> MPVDFTGYWKMLVNENFEEYLRALDVNVALR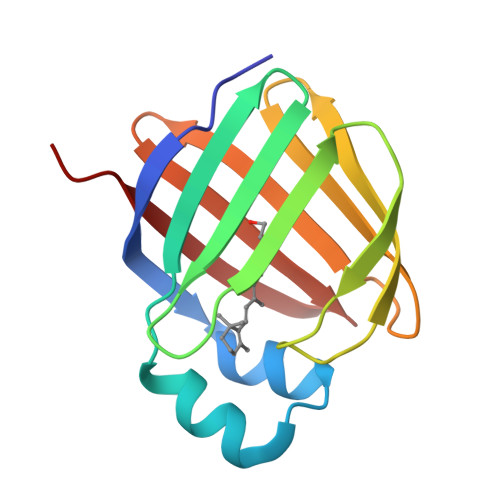KIANLLKPDKEIVQDGDHMIIRTLSTFRNYIMDFQVGKEFEEDLTGIDDRKCMTTVSWDGDKLQCVQKGEKEGRGWTQWIEGDELHLEMRVEGVVCKQVFKKVQ>CCAGTACUGG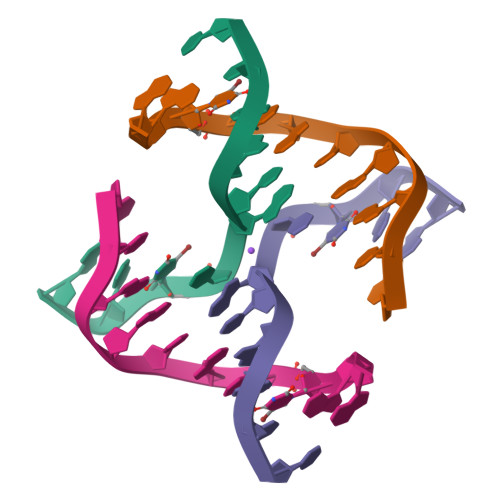[2x]> SNNALQTIINARLPGEEGLWQIHLQDGKISAIDAQSGVMPITENSLDAEQGLVIPPFVEPHIHLDTTQTAGQPNWNQSGTLFEGIERWAERKALLTHDDVKQRAWQTLKWQIANGIQHVRTHVDVSDATLTALKAMLEVKQEVAPWIDLQIVAFPQEGILSYPNGEALL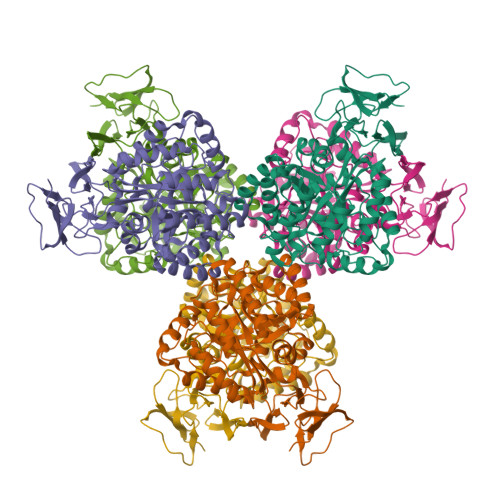EEALRLGADVVGAIPHFEFTREYGVESLHKTFALAQKYDRLIDVHCDEIDDEQSRFVETVAALAHHEGMGARVTASHTTAMHSYNGAYTSRLFRLLKMSGINFVANPLVNIHLQGRFDTYPKRRGITRVKEMLESGINVCFGHDDVFDPWYPLGTANMLQVLHMGLHVCQLMGYGQINDGLNLITHHSARTLNLQDYGIAAGNSANLIILPAENGFDALRRQVPVRYSVRGGKVIASTQPAQTTVYLEQPEAIDYKR>MDSIQAEEWYFGKITRRESERLLLNAENPRGTFLVRESETTKGAYCLSVSDFDNAKGLNVKHYKIRKLDSGGFYITSRTQFNSLQQLV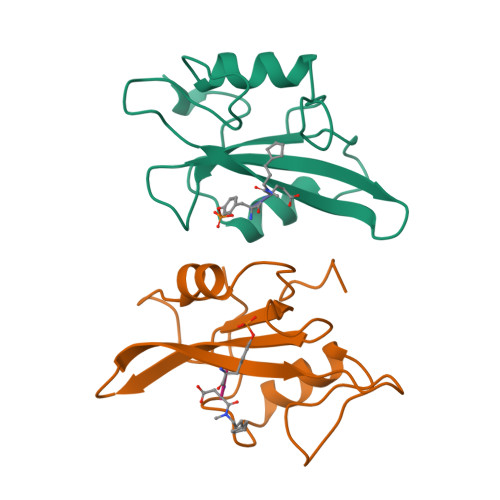AYYSKHADGLCHRLTTVCP[2x]>MRLREWLIAQIDSAEYPGLSWENAEKSMFRIPWKHAAKQDYRQNQDAALFKAWAMYKGKFQEGRDKADPSTWKTRLRCALNKSTDFQEVSERSQLDISEPYKVYRI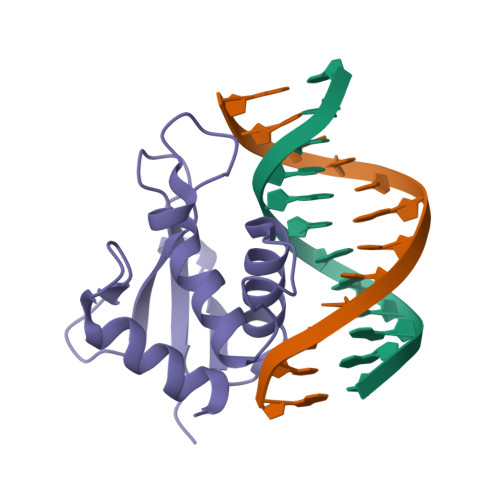LED[2x]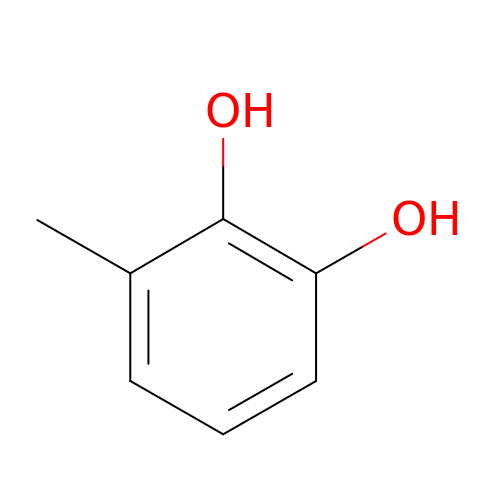3-METHYLCATECHOL | C7 H8 O2 | PGSWEKYNAOWQDF-UHFFFAOYSA-N> MREESTDECDGAIIGTAVKGHVAVHSDLSYWIESRYNDTWKLERAVFGEVKSCTWPETHTLWGDDVEESELIIPHTIAGPKSKHNRREGYKTQNQGPWDENGIVLDFDYCPGTKVTITEDCSKRGPSVRTTTDSGKLITDWCCRSCSLPPLRFRTENGCWYGMEIRPVMHDETTLVRSQVDAF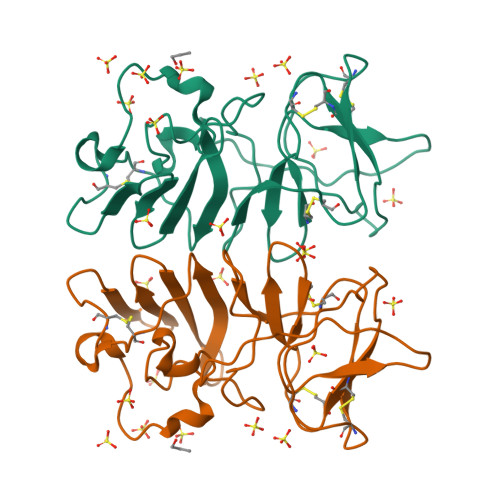KGEMVDPFSAGPSGDVSGHPGSPSQEVDGQIDHSCGFGGPTCADAWGYHLH>MRGSHHHHHHTDPQGDAAQKTDTSHHDQDHPTFNKITPNLAEFAFSLYRQLAHQSNSTNIFFSPVSIATAFAMLSLGTKADTHDEILEGLNFNLTEIPEAQIHEGFQELLRTLNQPDSQLQLTTGNFLFLSEGLKLVDKFLEDVKKLYHSEAFTVNFGDTEEAKKQINDYVEKGTQGKIVDLVKELDRDTVFALVNYIFFKGKWERPFEVKDTEEEDFHVDQVTTVKVPMMKRLGMFNIQHCKKLSSWVLLMKYLGNATAIFFLPDEGKLQHLENELTHDIITKFLENEDRRSASLHLPKLSITGTYDLKSVLGQLGITKVFSNGADLSGVTEEAPLKLS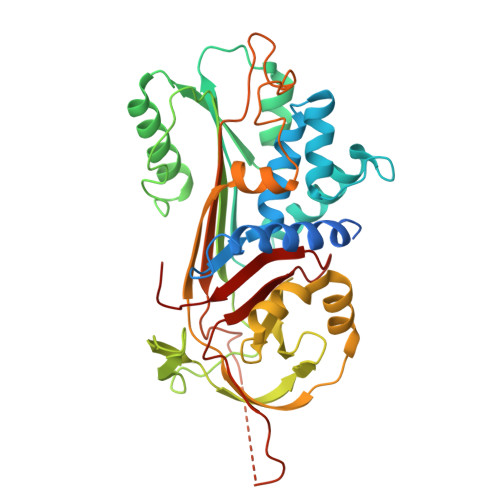KAVHKAVLTIDEKGTEAAGAMFLEAIPMSIPPEVKFNKPFVFLMIEQNTKSPLFMGKVVNPTQK[3x]> TPENIRFVFAAVK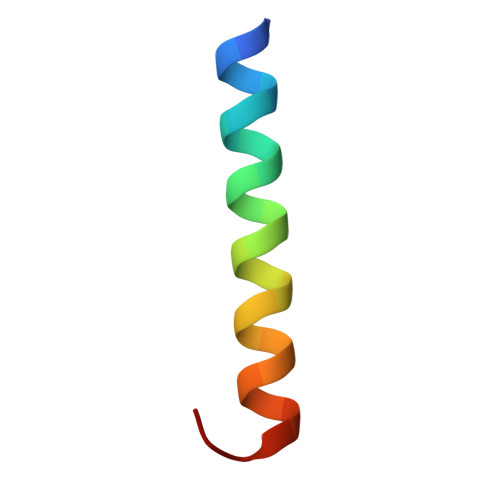DTILQLNLKEYNLV The GH45 family is composed mainly of β-1,4-endoglucanases from a number of organisms including plants, animals, bacteria and fungi. On the other hand, PcCel45A, a member of subfamily C, lacks one of the two catalytic residues and thus employs a distinct catalytic mechanism different from that of the GH45 subfamily A members. It has been recently proposed that PcCel45A utilizes an imidic acid form of asparagine residue as general base in a “Newton’s cradle” proton relay catalytic mechanism. Despite the same fold (double psi-β-barrel) and the homologous sequence, the PcCel45A structure is significantly different from HiEGV and MaCel45A.

The structure of the PcCel45A-cellobiose complex revealed a single cellobiose molecule within the active-site groove. In all cases cellobiose is located at the +1 and +2 subsites of the active sites. The residues Asp114, Met17, Gly131, Tyr67 and Asn92 in PcCel45A X-ray structure form direct hydrogen bonds with the cellobiose. At the +2 position, the amide nitrogen of Met17 (N) and the carbonyl oxygen of Gly131 (O) interact with O6’ of cellobiose, and possibly stabilize the ligand in the active site. Furthermore, the O2’ atom forms a hydrogen bond with the hydroxyl of the Tyr67 phenyl ring (2.9 Å). The Asn92 OD1 forms hydrogen bonds with O4 and O6 (2.7 and 3.3 Å) at the +1 position. Another carboxyl group (OD2) of the catalytic Asp114 side chain interacts with the non-reducing end of cellobiose (O4) at the +1 position (2.7 Å). The comparison between apo-PcCel45A structure and its complex with cellobiose reveals that the ligand binding induces a small conformational change in B1 and B5 strands, where the residues Met17 and Asp114 are respectively located. Closer examination of PcCel45A structure bound to cellobiose revealed that the Asp114 side chain in the PcCel45A structure is inserted in a hydrophobic environment and its carboxyl group forms a hydrogen bond to the O4 atom of the +1 subsite glucopyranosyl unit. In addition, simulations of the PcCel45A bound to the cellobiose (C2) molecule present in our crystallographic structure and occupying the +1 and +2 subsites, showed that it dissociates in a shorter time scale than C3.

> ATGGYVQQATGQASFTMYSGCGSPACGKAASGFTAAINQLAFGSAPGLGAGDACGRCFALTGNHDPYSPNYTGPFGQTIVVKVTDLCPVQGNQEFCGQTTSNPTNQHGMPFHFDICEDTGGSAKFFPSGHGALTGTFTEVSCSQWSGSDGGQLWNGACLSGETAPNWPSTACGNKGTAPS>[4x]MAGDPMITETQLTAIQTYALQKLAHDHSGHGRDHLQRVNRLARRLAKDEGANLNLTLAAAWLHDVIDDKLM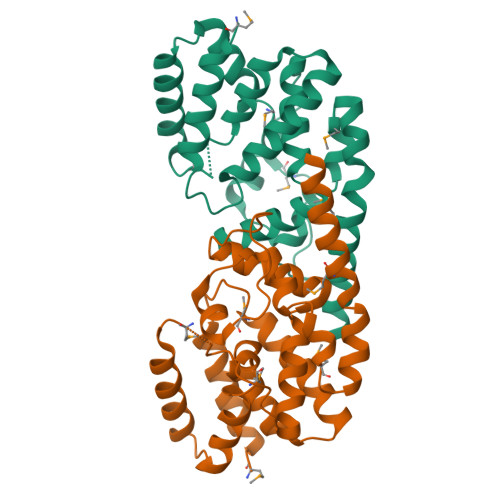ANPAKAHQDLIVQLNAQNVTADDQTAIFAIIDHMSFSKSFNGPQKLSLEGQVVQDADRLDAIGAIGIARALYYSGHVGEKIYDPAIAPREHMTREQYRHQPGTAINHFYEKLFKLAALMNTDTAKALAAHRTAVMHEFVDQFKAEWTADDKALEHHHHHH> GPTYVQALFDFDPQEDGELGFRRGDFIHVMDNSDPNWWKGACHGQTGM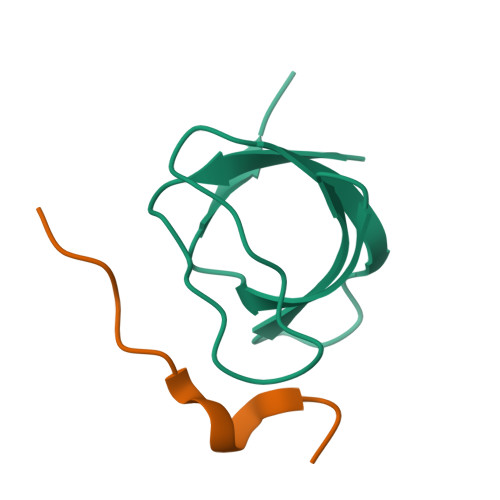FPRNYVTAVN;> IQPPPVNRNLKPDRK> ESNPDPTTYPDVELSPPPRISLRSLLTAQPVKNDHYDSHNYLSTHWELIDYKGKEYEKLRDGGTLVQFKVVGAAKCFAFLGKGTTDCKDTDHTVFNLIPT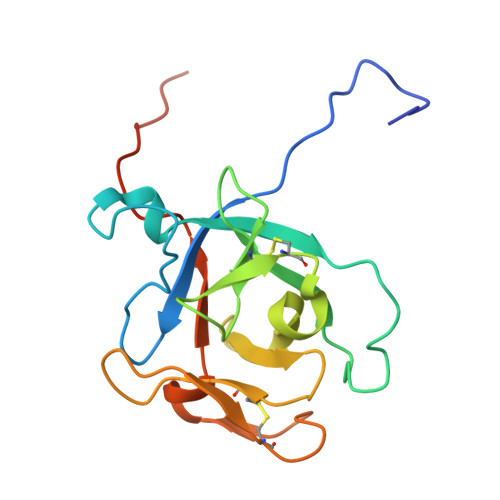NTGAFLIKDALLGFCITSHDFDDLKLEPCGGSVSGRTFSLAYQWGILPPFGPSKILIPPVRRNQGS> PP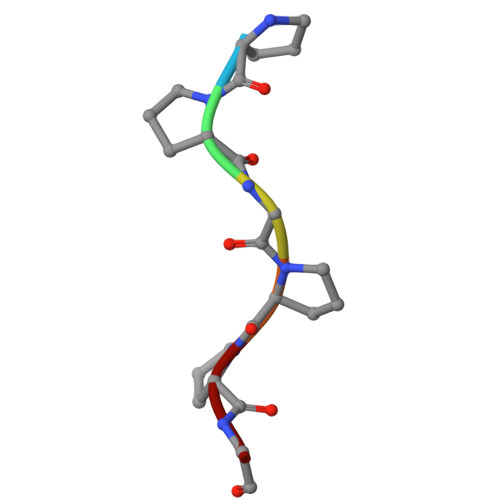GPPG> GPHMASMLEAKFEEASLFKRIIDGFKDCVQLVNFQCKEDGIIAQAVDDSRVLLVSLEIGVEAFQEYRCDHPVTLGMDLTSLSKILRCGNNTDTLTLIADNTPDSIILLFEDTKKDRIAEYSLKLMDIDADFLKIEELQYDSTLSLPSSEFSKI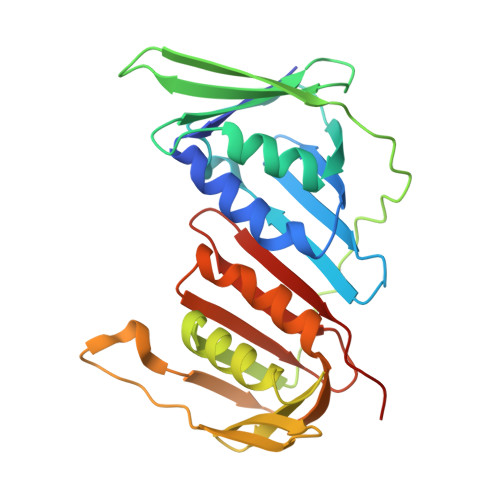VRDLSQLSDSINIMITKETIKFVADGDIGSGSVIIKPFVDMEHPETSIKLEMDQPVDLTFGAKYLLDIIKGSSLSDRVGIRLSSEAPALFQFDLKSGFLQFFLAPKFNDEE>MTVHKKQYKVAAVQAAPAFLDLEAGVAKAIGLIAQAAAEGASLVAFPEAWLPGYPWWIWLDSPAGGMRFVQRNFDNALEVGSEPFERLCRAAAQHKIYVVLGFTERSGGTLYLAQAIIDDCGRVVATRRKLKPTHVERSVYGEGDGSDLAVHDTTLGRLGALCCAEHIQPLSKYAMYAQHEQVHIAAWPSFSVYRGAAFQLSAQANNAASQVYALEGQCFVLAPCATVSKEMLDELIDSPAKAELLLEGGGFAMIYGPDGAPLCTPLAETEEGILYADIDLGVIGVAKAAYDPVGHYSRPDVLRLLVNREPMTRVHYVQ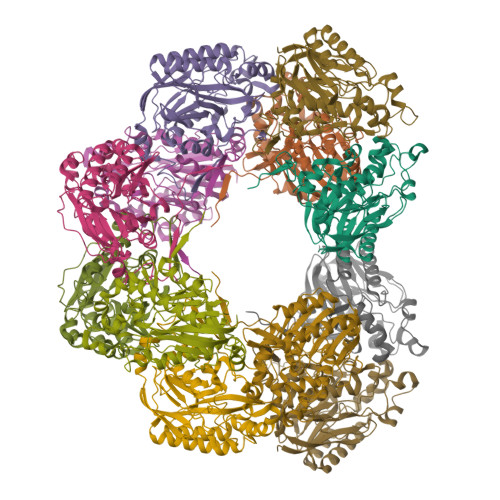PQSLPETSVLAFGAGADAIRSEENPEEQGDK[12x]N-methyl-N-[1-[4-(2-methylpyrazol-3-yl)phthalazin-1-yl]piperidin-4-yl]-4-nitro-2-(trifluoromethyl)benzamide | C26 H24 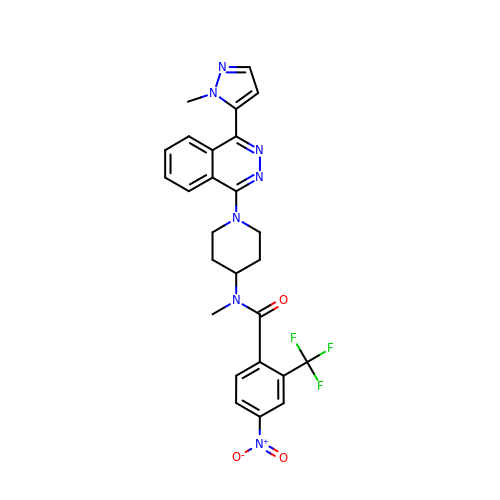F3 N7 O3 | ZDEZQXNVPSUJHK-UHFFFAOYSA-N> GSGQSLNPHNDYCQHFVDTGHRPQNFIRDVGLADRFEEYPKLRELIRLKDELIAKSNTPPMYLQADIEAFDIRELTPKFDVILLEPPLEEYYRETGITANEKCWTWDDIMKLEIDEIAAPR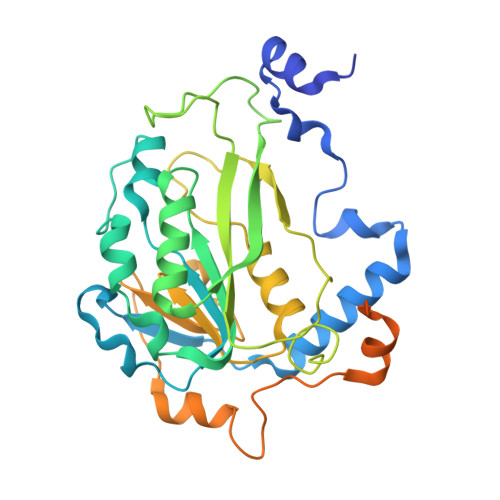SFIFLWCGSGEGLDLGRVCLRKWGYRRCEDICWIKTNKNNPGKTKTLDPKAVFQRTKEHCLMGIKGTVKPSTDGDFIHANVDIDLIITEEPEIGNIEKPVEIFHIIEHFCLGRRRLHLFGRDSTIRPGWLTVGPTLTNSNYNAETYASYFSAPNSYLTGCTEEIERLRPKSPPPKSKSDRGGGAPRGGGRGGTSAGRGRERNRSNFRGERGGFRGGRGGAHRGGFPPR>ARTFFVGGNFKLNGSKQSIKEIVERLNTASIPENVEVVICPPATYLDYSVSLVKKPQVTVGAQNAYLKASGAFTGENSVDQIKDVGAKWVILGQSERRSYFHEDDKFIADKTKFALGQGVGVILCIGETLEEKKAGKTLDVVERQLNAVLEEVKDWTNVVVAYEPVWAIGTGLAATPEDAQDIHASIRKFLASKLGDKA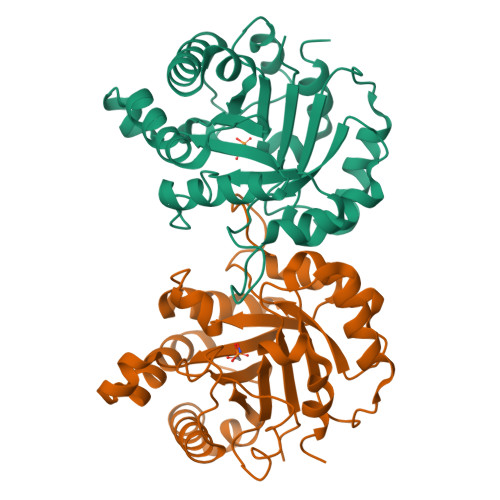ASELRILYGGSANGSNAVTFKDKADVDGFLVGGASLKPEFVDIINSRN[2x]>MSLDSDPDTLVVHTQLGTTAPGSPTYLAAVDRFREENPGVKIKNLVNGDDLAQVYETSRLARKEADVVMVNLYDKTLAWTDVGATVDVKPYLDDWGLRGRVLPAALADWTDDEGRVRAFPYFATNWPVAYNRALLDRAGVDAIPTTGDQLIAAARKLRAKGIAPVTVGGNDWTGQKLLAQIIQTFLSQDEARHVYSTGDFGVRGARLGIEYFAHLRDAGVFADKAQGLTSDSMTTQFNTEEAAVQSAMSSALAKVPEKVAGHTEVGGWPLADGAAHDGPTVIRAYTLIGFWISPNGVRKIEQ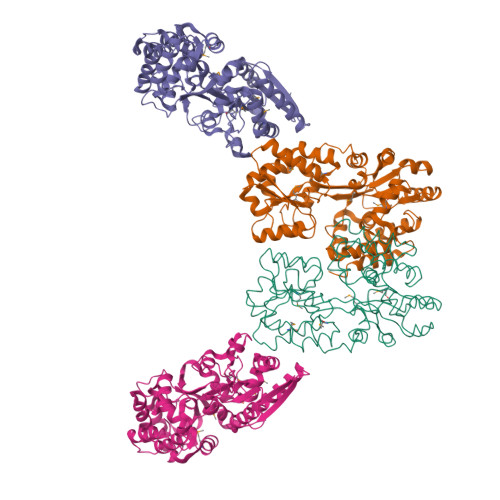VEKFLRFMYRPDVVARFVTESGRDMALRTDAVSTGFPLVGAAQRLGSEVSQVLLPDVYVPPAAAQPLITATSTSFTRGTSPARVRAALESAYRSVEGHHHHHH[4x]>[4x]MVSKLSQLQTELLA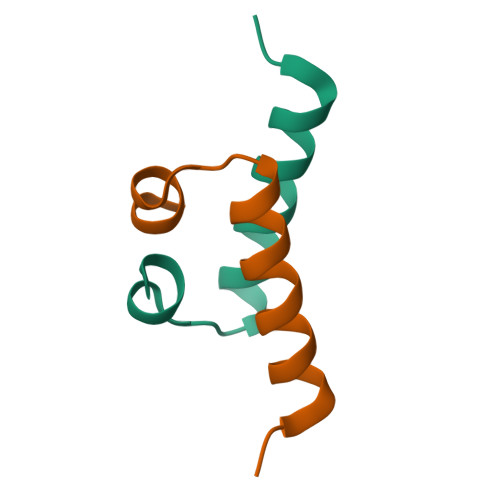ALLESGLSKEALIQALGE>GSLDLHGLHVDEALEHLMRV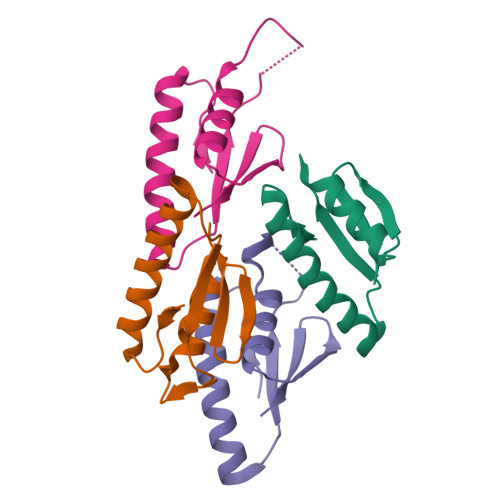LEKKTEEFKQNGGKPYLSVITGRGNHSQGGVARIKPAVIKYLISHSFRFSEIKPGCLKVMLK[4x]> MREYKLVVLGSGGVGKSALTVQFVQGIFVDEYDPTIEDSYRKQVEVDCQQCMLEILDTAGTEQFTAMRDLYMKNGQGFALVYSITAQSTFNDLQDLREQILRVKDTEDVPMILVGNKCDLEDERVVGKEQGQNLARQWCNCAFLESSAKSKINVNEIFYDLVRQINR;> PSKT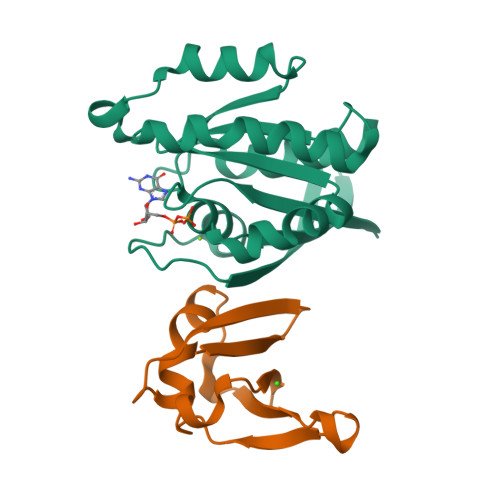SNTIRVFLPNKQRTVVRVRNGMSLHDCLMKKLKVRGLQPECCAVFRLLHEHKGKKARLDWNTDAASLIGEELQVDFL>GSAAAQDMVSPPPPIADEPLTVNTGIYLIECYSLDDKAETFKVNAFLSLSWKDRRLAFDPVRSGVRVKTYEPEAIWIPEIRFVNVENARDADVVDISVSPDGTVQYLERFSARVLSPLDFRRYPFDSQTLHIYLIVRSVDTRNIVLAVDLEKVGKNDDVFLTGWDIESFTAVVKPANFALEDRLESKLDYQLRISRQYFSYIPNIILPMLFILFISWTAFWSTSYEANVTLVVSTLIAFIAFNILVETNLPKTPYMTYTGAIIFMIYLFYFVAVIEVTVQHYLKVESQPARAASITRASRIAFPVVFLLANIILAFLFF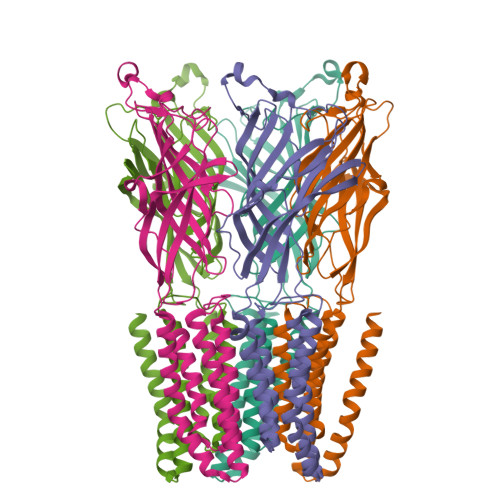GF[5x]5-(4-fluorophenyl)-~{N}-[[3-[(~{S})-(1-methylindazol-5-yl)-oxidanyl-methyl]phenyl]methyl]-2,3-bis(oxidanyl)benzamide | C29 H24 F N3 O4 | 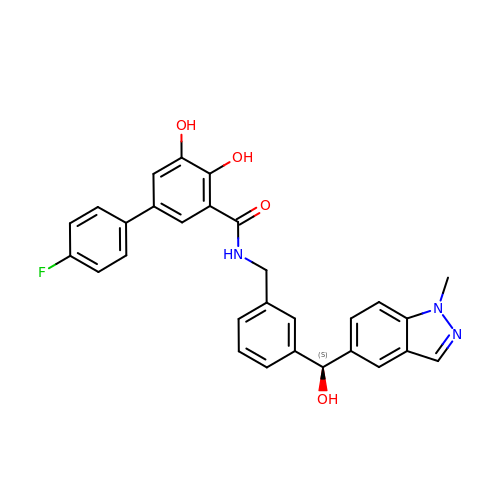AYTCJOWSEKPFCS-MHZLTWQESA-N>[3x]MSVTRLTSSLVRWKSKLANAIQRSLSSKMEESLSVLDFGAVADYNPTTKTGTDNTQAFRNAVAAAIAQNIRNVYAPGGPSAYMTTGEINLGGEGFTGGEGSRDVWRGITQGVHFFGDGPYSTIIAFNPPNTDAPCFSARGGWGTHSPRALSKLAIEPVNWADYNATSSGTGVLLQGCCFVPVTDVHI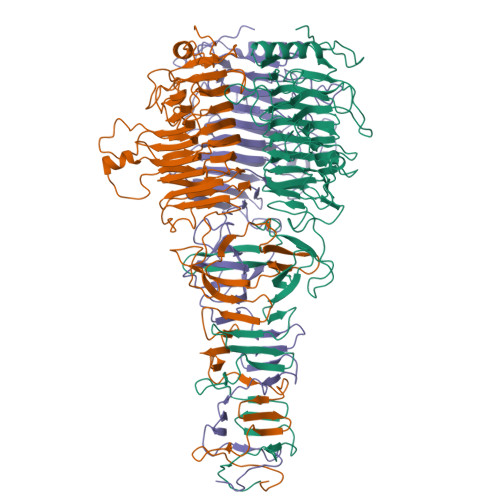GRFHRGIHFWNKLQGTDDPTNTFTKGDFTEFNRITRVRVFNCDIDVDYQVSLGNNSFHGNSFTDCMCQINSYGGIGMRMWDDGSRNAIRPSSLPYEYIANVYNNKHEINWFGSDARTCYLMHIDKAQGRGCNGDMTVEAAVTLRAIGQYWYQSFGSLHSISAINTVVDGDTDTATRPVAFMWMNSAYPQVNFDGTDPLLTSGLTPRQYDLNNSGNTGMELLNIRGANTGAIWSIQNGAALGWILGRRAQADSRKGTRSVWQFSYNGEVIKSVSAANVGLQNSTGAGFGMLGDTLLRPYAASTISLGSPTYPFTRLRTTDWTVDTNGIVPVQDGIKNIGSSSLRVGTVFAATGTINTSDARLKTEVRPFTSEEILAAKALSEEIGMYQWVASIESKGDNAREHCGLTVQRAMEVMQQHGLDPFNYGFICHDVWDEVVEVSDETGEVISSTPAGDRYSFRFDQLSLFISRGIEARMSELESRM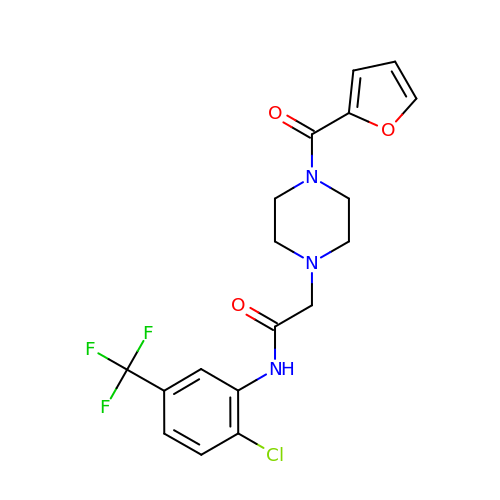N-[2-chloro-5-(trifluoromethyl)phenyl]-2-[4-(furan-2-carbonyl)piperazin-1-yl]acetamide | C18 H17 Cl F3 N3 O3 | OXKNHBBDOIMFFQ-UHFFFAOYSA-N>[4x]ADLESLYRAMPSIKKLVDEGKLTEKDAEKVYEIWRNMEAIYKQASLLWYNTVDLLL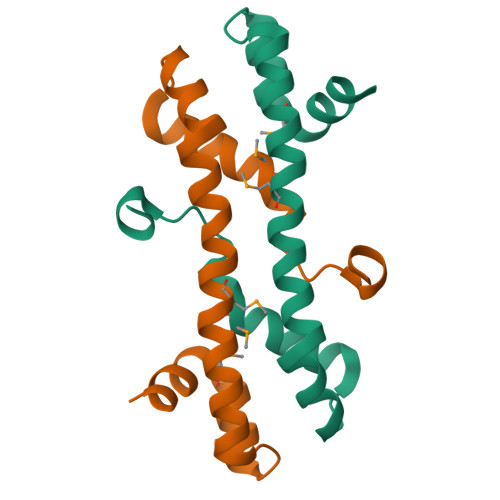KRIGLSEKEREEIFYEMVRPYFRLFSREEVFPKEVLEGKL> MADYKDDDDKSGPDEVDASGRMNWVQRKIYLYNVTFGLYMLDWWERYLFNSLVVVLMWFVLYNGTRYFSELF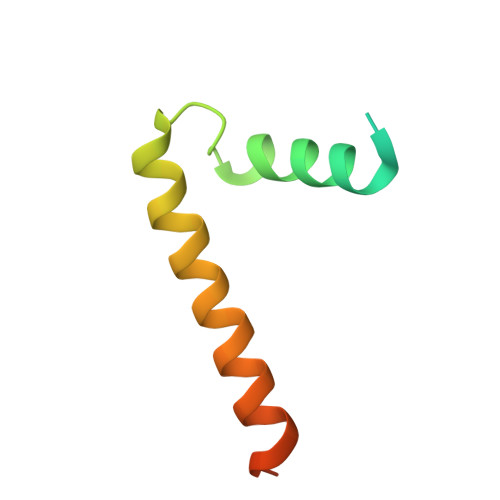QRHLT>[2x]GPGSGMTDEKTATARAKVVDWCNELVIASPSTKCELLAKVQETVLGSCAELAEEFLESVLSLAHDSNMEVRKQVVAFVEQVCKVKVELLPHVINVVSMLLRDNSAQVIKRVIQACGSIYKNGLQYLCSLMEPGDSAEQAWNILSLIKAQILDMIDNENDGIRTNAIKFLEGVVVLQSFADEDSLKRDGDFSLADVPD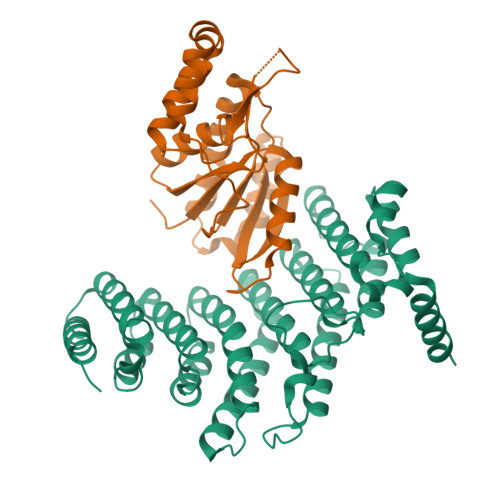HCTLFRREKLQEEGNNILDILLQFHGTTHISSVNLIACTSSLCTIAKMRPIFMGAVVEAFKQLNANLPPTLTDSQVSSVRKSLKMQLQTLLKNRGAFEFASTIRGMLVDLGSSTNEIQKLIPKMDKQEMARRQKRILENAAQ;>[2x]GPGSGMTDPSKLAVAVVDSSNMNRSMEAHNFLAKKGFNVRSYGTGERVKLPGMAFDKPNVYEFGTKYEDIYRDLESKDKEFYTQNGLLHMLDRNRRIKKCPERFQDTKEQFDIIVTVEERVYDLVVMHMESMESVDNRPVHVLNVDVVNNAEDALMGAFVITDMINMMAKSTDLDNDIDELIQEFEERRKRVILHSVLFY>MAHHHHHHMLKDTYPYYLANEAVYANTDLEVTDKFSGKVATRVALADAQAIDAAIGAAVDAVKPMRELPAYRRQAVLDHCVARFRERFDELAEALCIEAGKPINDSRGEVTRLIDTFRVASEEAVRIDGEVLNLEISARAQGYTGYTRRVPIGPCSFISPFNFPLNLAAHKVAPALAAGCPFVLKPASRTPVGALIIAEVLAETNLPKGAFSVLPAHRDGADLFTTDERFRLLSFTGSPAVGWALKEKAGKKKVVLELGGNAAAIVDADQFEQLDYVVDRLAFGAYYQSGQSCIGVQRILVHASLYDTLRDKLVAKTRSLKMGDPKDPSTFVGPMISESESRRLSGWMDAAVAAGAKIIAGGKVDGAMFEATLLEDVGREQDLYRKEAFGPVAILEKFDRFDDALARVNDSDFGLQAGVFTDSLTHAQRAWDELEVGGVVINDVPSFRVDNMPYGGVKDSGLGREG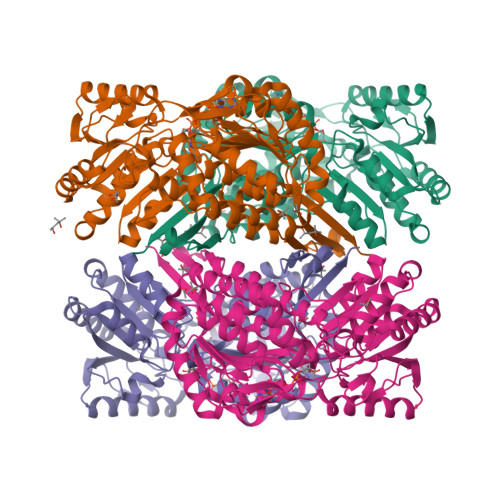IRYAIEDMTEPRLMVVRRR[4x]> MASFL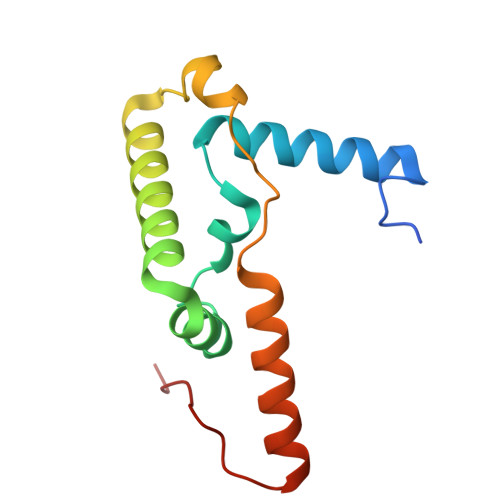QRLVDPRKNFLARMHMKSVSNRLRRYGLRYDDLYDPLYDLDIKEALNRLPREIVDARNQRLMRAMDLSMKHEYLPDNLQAVQTPFRSYLQDMLALVKRERAEREALGALPLYQRTIP> M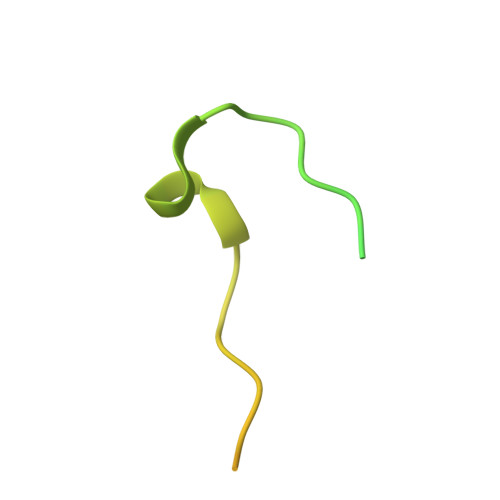GAQVSRQNVGTHSTQNSVSNGSSLNYFNINYFKDAASSGASRLDFSQDPSKFTDPVKDVLEKGIPTLQ> MAERQEEQRGSPPLRAEGKADAEVKLILYHWTHSFSSQKVRLVIAEKALKCEEHDVSLPLSEHNEPWFMRLNSTGEVPVLIHGENIICEATQIIDYLEQTFLDERTPRLMPDKESMYYPQVQHYRELLDSLPMDAYTHGCILHPELTVDSMIPAYATTRIRSQIGNTESELKKLAEENPDLQEAYIAKQKRLKSKLLDHDNVKYLKKILDELEKVLDQVETELQRRNEETP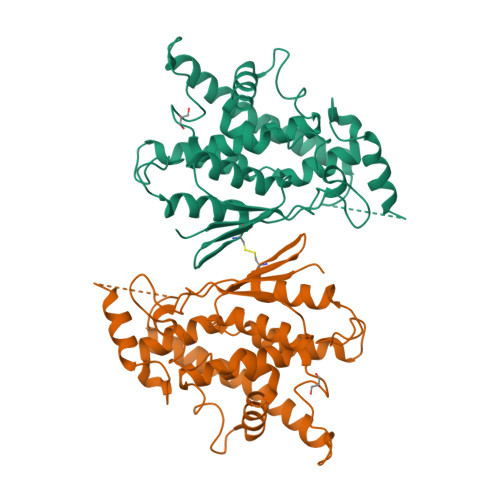EEGQQPWLCGESFTLADVSLAVTLHRLKFLGFARRNWGNGKRPNLETYYERVLKRKTFNKVLGHVNNILIS>GEKKECWSWESYLEEQKAITAPVSLFQDSQAVTHNKNGFKLGMKLEGIDPQHPSMYFILTVAEVCGYRLRLHFDGYSECHDFWVNANSPDIHPAGWFEKTGHKLQPPKGYKEEEFSWSQYLRSTRAQAAPKHLFVSQSHSPPPLGFQVGMKLEAVDRMNPSLVCVASVTDVVDSRFLVHFDNWDDTYDYWCDPSSPYIHPVGWCQKQGKPLTPPQDYPDPDNFCWEKYLEETGASAVPTWAFKVRPPHSF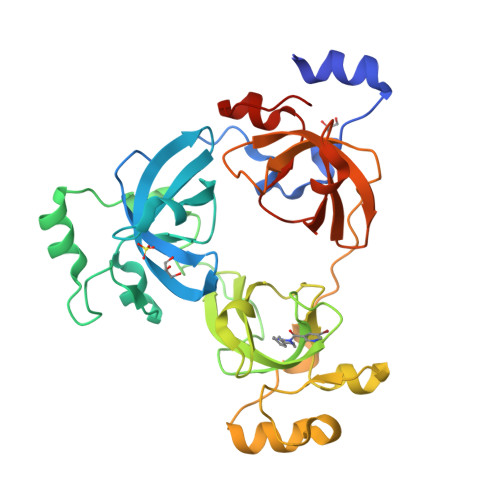LVNMKLEAVDRRNPALIRVASVEDVEDHRIKIHFDGWSHGYDFWIDADHPDIHPAGWCSKTGHPLQPPLGPRE[3x]> MPSKVDICNRALSNTGTDITIASLTEKSKEARLCQQWYDATLASLLRTYQWAFAQRRVTLA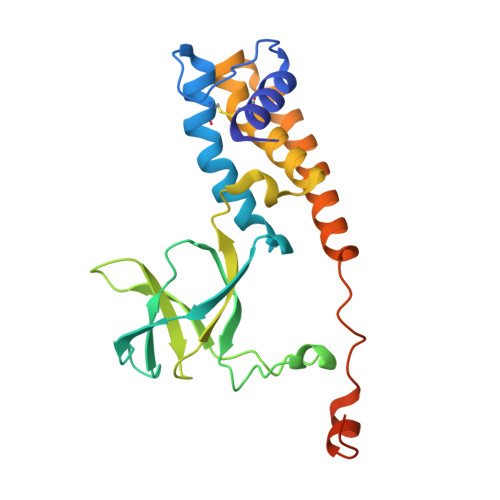LIGVGPAGWRHKYRYPTDAITIHDVFTADTYPDGASEFTDGRYRQIFQIASDGEGGRLVLANCEDAMCRYTSDIEDPNLMPPDFSTALEMMLAKNIAMPMTGNPGLMTVLAQQAASLVSDAIARDQNEGYRNPLPYASWTRANIGDSYPDDDHLPHRGGRR> METAPKPVGPYSQAVESGCFMFVSGQIPINPETGALEEGGFKESAKRALDNLKAIVEGAGYSMDDIVKVTVYITDISRFSE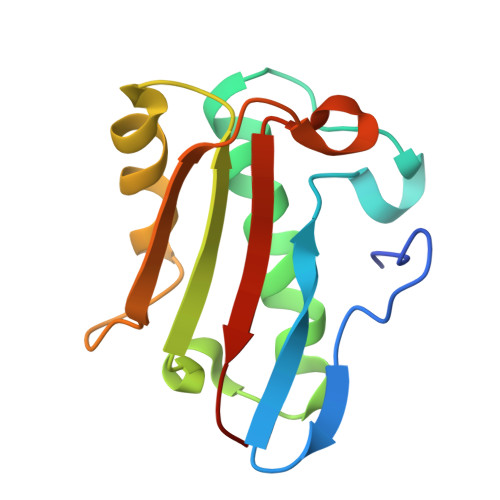FNEVYREYFNRPYPARAVVGVAALPLGAPLEVEAVLYTCRRK> MKTLVHVASVEKGRSYEDFQKVYNAIALKLREDDEYDNYIGYGPVLVRLAWHISGTWDKHDNTGGSYGGTY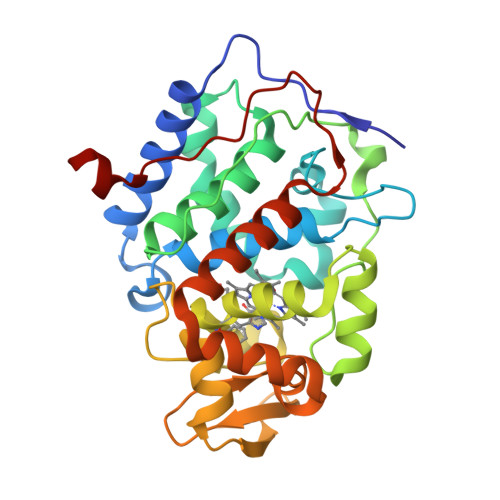RFKKEFNDPSNAGLQNGFKFLEPIHKEFPWISSGDLFSLGGVTAVQEMQGPKIPWRCGRVDTPEDTTPDNGRLPDADKDAGYVRTFFQRLNMNDREVVALMGAHALGKTHLKNSGYEGPGGAANNVFTNEFYLNLLNEDWKLEKNDANNEQWDSKSGYMMLPTDYSLIQDPKYLSIVKEYANDQDKFFKDFSKAFEKLLEDGITFPKDAPSPFIFKTLEEQGL> 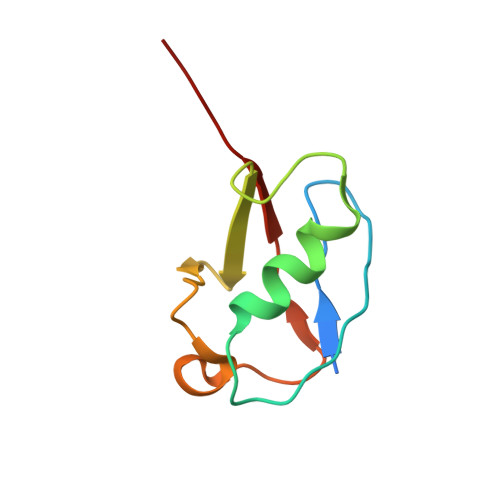MGEGEYIKLKVIGQDSSEIHFKVKMTTHLKKLKESYCQRQGVPMNSLRFLFEGQRIADNHTPKELGMEEEDVIEVYQEQTGG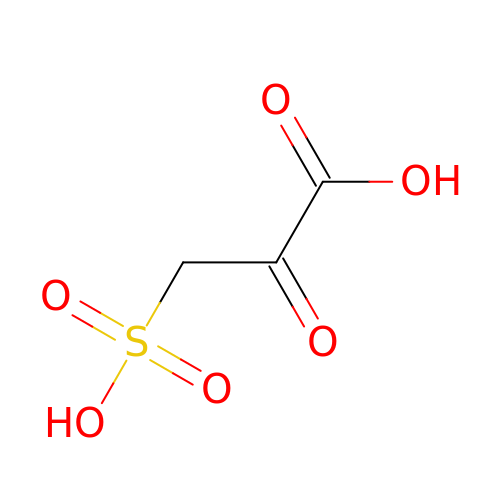SULFOPYRUVATE | C3 H4 O6 S | BUTHMSUEBYPMKJ-UHFFFAOYSA-N>GAMDVLSEKIWDYHNKVSQTDEMLQRKLHLRDMLYTAISPVFPLSGLYVVGSSLNGFGNNSSDMDLCLMITNKDLDQKNDAVVVLNLILSTLQYEKFVESQKLILAKVPILRINFAAPFDDITVALNANNSVAIRNTHLLCYYSSYDWR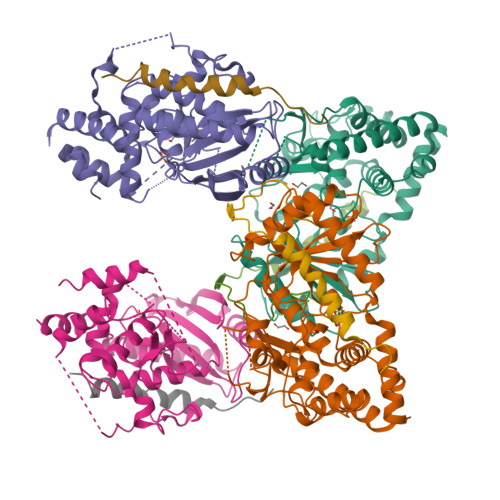VRPLVSVVKEWAKRKGINDANKSSFTSYSLVLMVIHFLQCGPTKVLPNLQQSYPNRFSNKVDVRTLNVTMALEEVADDIDQSLSEKTTLGELLIGFLDYYANEFNYDRDAISIRQGRRVERASISNPHFWRSQWRCVCIEEPFTNSNTAHSIYDEMVFEAIKKAFREAHGELQHNHDLDKLMECEPIKA[4x];>[4x]TLFDNHPVQQYSGFNPIDFRFDDYVEGAKRFDNLANLIRSSTPTDPFANYQKPCESTSTSRSRTNSAKDQKHGP1-{3-[AMINO(IMINO)METHYL]PHENYL}-N-[4-(1H-BENZIMIDAZOL-1-YL)-2-FLUOROPHENYL]-3-(TRIFLUOROMETHYL)-1H-PYRAZOLE-5-CARBOXAMIDE | C25 H17 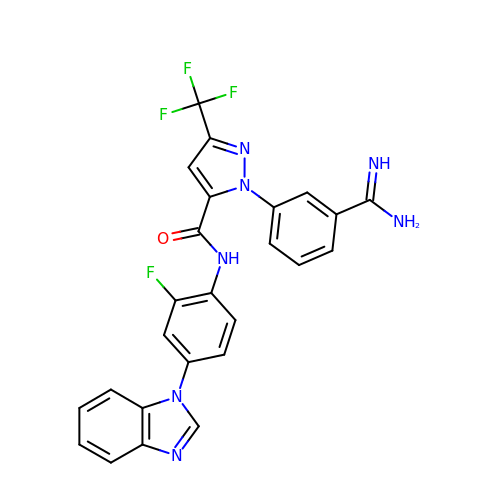F4 N7 O | TWBHVKYRNOGUJS-UHFFFAOYSA-N CHLOROACETONE | C3 H5 Cl O | 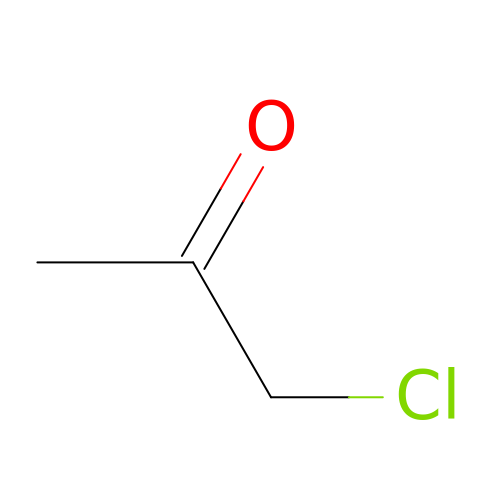BULLHNJGPPOUOX-UHFFFAOYSA-N>MKKGHHHHHHGS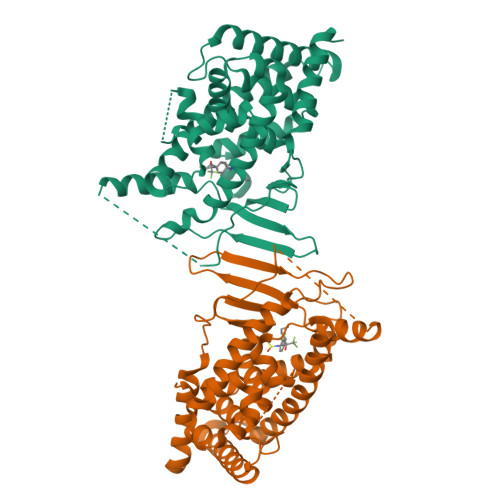ERTGTQPLGVQGLTEEQRMMIRELMDAQMKTFDTTFSHFKNFRLPGVLSSGCELPESLQAPSREEAAKWSQVRKDLCSLKVSLQLRGEDGSVWNYKPPADSGGKEIFSLLPHMADMSTYMFKGIISFAKVISYFRDLPIEDQISLLKGAAFELCQLRFNTVFNAETGTWECGRLSYCLEDTAGGFQQLLLEPMLKFHYMLKKLQLHEEEYVLMQAISLFSPDRPGVLQHRVVDQLQEQFAITLKSYIECNRPQPAHRFLFLKIMAMLTELRSINAQHTQRLLRIQDIHPFATPLMQELFGITGSSGGSGGSSHSSLTERHKILHRLLQEGSPSDITTLSVEPD[2x]> MAIGEFMVSLPRMVYPQPKVLTPCRKDVLVVTPWLAPIVWEGTFNIDILNEQFRLQNTTIGLTVFAIKKYVAFLKLFLETAEKHFMVGHRVHYYVFTDQPAAVPRVTLGTGRQLSVLEVRAYKRWQDVSMRRMEMISDFCERRFLSEVDYLVCVDVDMEFRDHVGVEILTPLFGTLHPGFYGSSREAFTYERRPQSQAYIPKDEGDFYYGGAFFGGSVQEVQRLTRACHQAMMV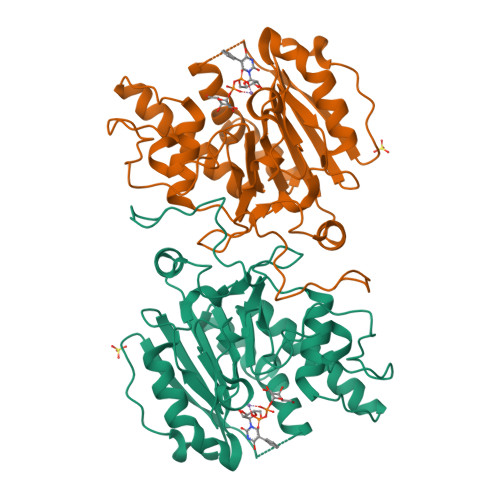DQANGIEAVWHDESHLNKYLLRHKPTKVLSPEYLWDQQLLGWPAVLRKLRFTAVPKNHQAVRNP>MLSSTKEYLQALRDGKYLLFLQWPKFIAEYYGKSDKNQEADEMVSLLIFEWLNNGFCLDDIKKFAILYAVHEMESRPLREGLSYALTTISIALFPCMVYLTNNLQEHYITSKKLSSKEVLQLMTMNNAYLEKQRFVEFLGQEQDKFFTWVKEADSSAVSKAFDQIYSVTYLKYLIEDYLSLLESA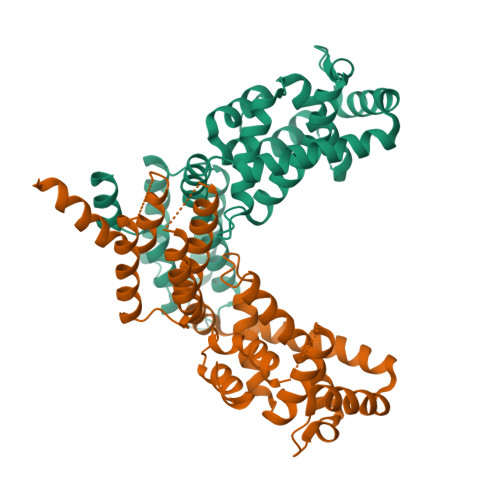HLPTDQLKSSRISLVVRLAKYLHEQTELTQDVHDEIAVYVKKLWEMQPAEFEEEFLKKISPLPFIDNTVRILTGLSARFFSILQPPSPPLNINSDTDKNPKV[4x]> MRGIEITITMQSDWHVGTGMGRGELDSVVQRDGDNLPYIPGKTLTGILRDSCEQVALGLDNGQTRGLWHGWINFIFGDQPALAQGAIEPEPRPALIAIGSAHLDPKLKAAFQGKKQLQEAIAFMKPGVAIDAITGTAKKDFLRFEEVVRLGAKLTAEVELNLPDNLSETNKKVIAGILASGAKLTERLGGKRRRGNGRCELKFSGYSDQQIQWLKDNYQSVDQPPKYQQNKLQSAGDNPEQQPPWHIIPLTIKTLSPVVLPARTVGNVVECLDYIPGRYLLGYIHKTLGEYFDVSQAIAAGDLIITNATIKIDGKAGRATPFCLFGEKLDGGLGKGKGVYNRFQESEPDGIQLKGERGGYVGQFEQEQRNLPNTGKINSELFTHNTIQDDVQRPTSDVGGVYSYEAIIAGQTFVAELRLPDSLVKQITSKNKNWQAQLKATIRIGQSKKDQYGKIEVTSGNSADLPKPTGNNKTLSIWFLSDILLRGDRLNFNATPDDLKKYLENALDIKLKERSDNDLICIALRSQRTESWQVRWGLPRPSLVGWQAGSCLIYDIESGTVNAEKLQELMITGIGDRCTEGYGQIGFNDPLLSASLGKLTAKPKASNNQSQNSQSNPLPTNHPTQDYARLIEKAAWREAIQNKALALASSRAKREEILGIKIMGKDSQPTMTQLGGFRSVLKRLHSRNNRDIVTGYLTALEQVSNRKEKWSNTSQGLTKIRNLVTQENLIWNHLDIDFSPLTITQNGVNQLKSELWAEAVRTLVDAIIRGHKRDLEKAQENESNQQSQGAA;> MPAGGRLMKNLYHYHQYEITLESAVDSCKNHLQAAIGLLYSPQKCELVKLDNSGKLVDSYNRLKFNNLGVFEARFFNLNCELRWVNESNGNGTAVLLSESDITLTGFEKGLQEFITAIDQQYLLWGEPAKHPPNADGWQRLAEARIGKLDIPLDNPLKPKDRVFLTSEEYIAEVDDFGNCAVIDERLIKLEVK;> MAHHHHHHVGTENLYFQGFLVLIETSGNQHFIFSTNKLRENIGASELTYLATTEILFQGVDRVFQTNYYDQWSDTNSLNFLADSKLNPAIDDPKNNADIEILLATSGKAIALVKEEGKAKQLIKEVTKQALINAPGLEIGGIYVNCNWQDKLGVAKAVKEAHKQFEVNRAKRAGANGRFLRLPIAAGCSVSELPASDFDYNADGDKIPVSTVSKVKRETAKSAKKRLRSVDGRLVNDLAQLEKSFDELDWLAVVHADGNGLGQILLSLEKYIGEQTNRNYIDKYRRLSLALDNCTINAFKMAIAVFKEDSKKIDLPIVPLILGGDDLTVICRGDYALEFTREFLEAFEGQTETHDDIKVIAQKAFGVDRLSACAGISIIKPHFPFSVAYTLAERLIKSAKEVKQKVTVTNSSPITPFPCSAIDFHILYDSSGIDFDRIREKLRPEDNTELYNRPYVVTAAENLSQAQGYEWSQAHSLQTLADRVSYLRSEDGEGKSALPSSQSHALRTALYLEKNEADAQYSLISQRYKILKNFAEDGENKSLFHLENGKYVTRFLDALDAKDFFANANHKNQGE;> MARKVTTRWKITGTLIAETPLHIGGVGGDADTDLALAVNGAGEYYVPGTSLAGALRGWMTQLLNNDESQIKDLWGDHLDAKRGASFVIVDDAVIHIPNNADVEIREGVGIDRHFGTAANGFKYSRAVIPKGSKFKLPLTFDSQDDGLPNALIQLLCALEAGDIRLGAAKTRGLGRIKLDDLKLKSFALDKPEGIFSALLDQGKKLDWNQLKANVTYQSPPYLGISITWNPKDPVMVKAEGDGLAIDILPLVSQVGSDVRFVIPGSSIKGILRTQAERIIRTICQSNGSEKNFLEQLRINLVNELFGSASLSQKQNGKDIDLGKIGALAVNDCFSSLSMTPDQWKAVENATEMTGNLQPALKQATGYPNNISQAYKVLQPAMHVAVDRWTGGAAEGMLYSVLEPIGVTWEPIQVHLDIARLKNYYHGKEEKLKPAIALLLLVLRDLANKKIPVGYGTNRGMGTITVSQITLNGKALPTELEPLNKTMTCPNLTDLDEAFRQDLSTAWKEWIADPIDLCQQEAA;> MTVGTLGVVGSAKNLKLQLSFINTRQQYVQITLFERNSFKVAEEEFSTELVEIIKTALPTLKNKKVEFEEDGDQIKQIREKGQAWVGAAEQIAPYVLPSGNITETPRNVNASNFHNPYNFVPALPRDGITGDLGDCAPAGHSYYHGDKYSGRIAVKLTTVTPLLIPDASKEEINNNHKTYPVRIGKDGKPYLPPTSIKGMLRSAYEAVTNSRLAVFEDHDSRLAYRMPATMGLQMVPARIEGDNIVLYPGTSRIGNNGRPANNDPMYAAWLPYYQNRIAYDGSRDYQMAEHGDHVRFWAERYTRGNFCYWRVRQIARHNQNLGNRPERGRNYGQHHSTGVIEQFEGFVYKTNKNIGNKHDERVFIIDRESIEIPLSRDLRRKWRELITSYQEIHKKEVDRGDTGPSAVNGAVWSRQIIADESERNLSDGTLCYAHVKKEDGQYKILNLYPVMITRGLYEIAPVDLLDETLKPATDKKQLSPADRVFGWVNQRGNGCYKGQLRIHSVTCQHDDAIDDFGNQNFSVPLAILGQPKPEQARFYCADDRKGIPLEDGYDRDDGYSDSEQGLRGRKVYPHHKGLPNGYWSNPTEDRSQQAIQGHYQEYRRPKKDGLEQRDDQNRSVKGWVKPLTEFTFEIDVTNLSEVEL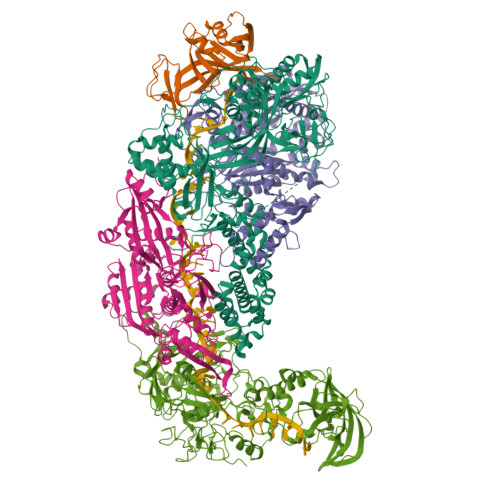GALLWLLTLPDLHFHRLGGGKPLGFGSVRLDIDPDKTDLRNGAGWRDYYGSLLETSQPDFTTLISQWINAFQTAVKEEYGSSSFDQVTFIKASGQSLQGFHDNASIHYPRSTPEPKPDGEAFKWFVANEKGRRLALPALEKSQSFPIKPS> GTNSKYITALKRSEGQLRGIQKMIEGDRDCADIVTQLTAVRSSVERVIEMIIT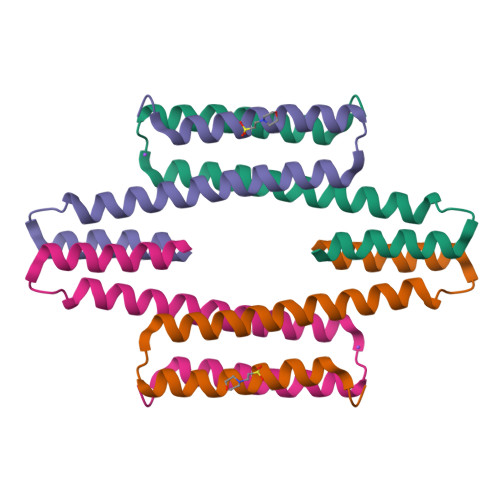EALTECINQPLDDSEAQKERLEKAIRYLIKRK>[2x]MTAITLHGPHQGPPQQPGQFQINHGQPGGSHNMNAQYAHHHPHHPVHLTRPSAGLISVASSPARNPGAFMRQTTLAISHLQAQYAEASGIQQDGYTGMRSMPPSAAYAAPTRPAQPITNGISEAVPPVQIHRRPSSAPSDQQESVNPASQINCGQDEDQEQSGPSGAVGKLAKPPLLRSKSERGLRHEQDESLDDEQYAYGARHGFEEAYQSEDIIS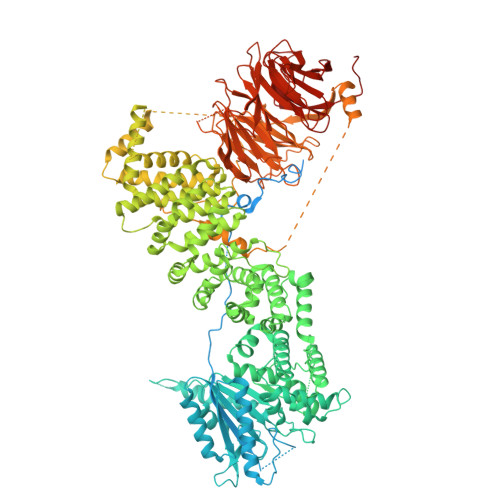QLANNWYMYFTDKRHETTGKPKSPTFEIQDWRMRDRLKTVSAAIAVCLNIGVEPPDQLRTNPGAKLEAWQDPTIPPVSKALENIGKALQSQYETLAIRTRCKQYLDPSIEETKKFCISLRRNAKDERVLFHYNGHGVPKPTASGEIWVFNKNYTQYIPVSLYDLQQWLQAPTIFVWDCSEAGNILKNYHKFVERHEKEEEEQAAKDPSYEKVNFRPYIHLAACASKENLPTNPMLPADLFTCCLTTPIEMALWFFVLQNPLKTKLTPERARKLGGRLQERRTPLGELNWIFTAITDTIAWTTLPRDLFRKFFRQDLMVAALFRNFLLAQRIMPVYGCHPQSYPELPDTRRHPLWEAWDHAVDMALAQLPMLERKERENIPYDYVPSTFFTEQLTAFEIYLTRGDAAAQKPPEQLPVVLQVLLSQQHRLRALILLGRFLDLGPWAVQLALSIGIFPYVLKLLQSAAQELKPVMVFIWTRILAVDISCQQDLIKDNGYTYFSSIMRPNETIPVVGLSVIDEHKAMCAFILSMLCKGFKTGQVVCNSTEIMTSCLYHTEHPDNPLLRQWSCLCISQLWKDFNEAKWRGIRENALQKLAALARDSCPEVRAAMIHAMTTFLGIPEVTDEVARLEEGIAWALLEMATDGSPIVRKELLVFWSVFVLRYENKFLVAAYEQLLEEKEYMLYPPPEDGLEHKMGLHYARPENREKDGTIKPSAYGVAHDSLYAAIWKHLCIMSVDPHPEVQRDATTIVDYIHHALLHSPVGTQAQTLMDEILRRASKVSRGDNSQRSSAAGTRAAPAQPMPSAGLLKRTASYLFGPLLGVTSDGSSTSSVSSTPTSAPGMNRSSSQRSRKGLNAANVLPEKPDQVAPPAAYHVAPEPLSPGYQERKPKEMPTLPLVSTFLEWSTEYFREPQMKPPEAEEPGSHEYNQRLWRRSRNEAVLRETQPQKLYARTHRWNNQIGLINNGTQPSKMTFHQFENCVAVADDGNTITVWDWKTNARLSRFSNGNPEGTKISDLCFINEDDQALLMTGSSDGVIRIYNNYDSDERVELASAWRALTHMVPSNVNSGMVFEWLQVNGRVLVAGDERVIRIWSAGQEICTHEIPARSGSCVTSLTSDQMTGNIFVAGFGDGAIRVFDSRLRPHEAMVRKWKDDARQWVRSVHMQRGGQRELLSASRNGKISLWDIRMDQPLKTFQSTKEILRTASTHEHLPVFAVGTSAHMVKVFDFDGNELTRLEPYSNFLQGSKASPIATTAFHPHRMILGCASRGDNYISLYSCSNERVPNLV>MPGLFLTLEGLDGSGKTTQARRLAAFLEAQGR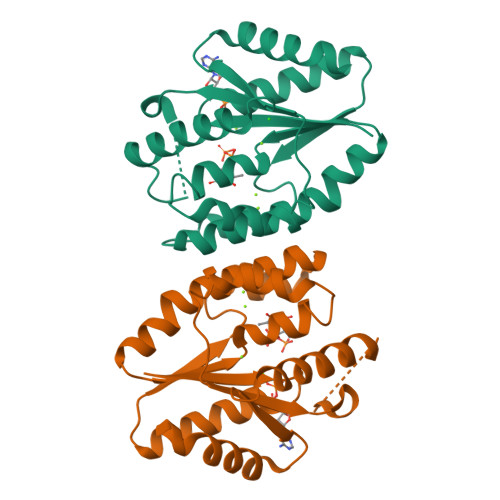PVLLTREPGGGLPEVRSLLLTQELSPEAEYLLFSADRAEHVRKVILPGLAAGKVVISDRYLDSSLAYQGYGRGLPLPWLREVAREATRGLKPRLTFLLDLPPEAALRRVRRPDRLEGLGLEFFRRVREGYLALARAEPGRFVVLDATLPEEEIARAIQAHLRPLLP[2x]> MGHHHHHHGSGSTNINLFSSYQLGELELPNRIVMAPLTRSRAGEGNVPHQLNAIYYGQRASAGLIIAEATQVTPQGQGYPHTPGIHSPEQVAGWKLVTDTVHQQGGRIFLQLWHVGRISHPDLQPDGGLPVAPSAIAPKGEVLTYEGKKPYVTPRALDTSEIPAIVEQYRQGAANALAAGFDGVEIHAANGYLIDQFLRDGTNKRTDEYGGAIENRARLLLEVTEAITSVWDSQRVGVRLSPLTTLNGCVDSHPLETFGYVAQALNRFNLSYLHIFEAIDADIRHGGTVVPTSHLRDRFTGTLIVNGGYTREKGDTVIANKAADLVAFGTLFISNPDLPERLEVNAPLNQADPTTFYGGGEKGYTDYPFLAVANK

To generalize this engineering approach for crystal contacts, a non-ADH-homologous enzyme was selected to apply the established strategies to the Nostoc sp. PCC 1720 ene reductase (NostocER). This oxidoreductase from the old yellow enzyme family (OYE, EC 1.6.99.1) catalyzes the trans-hydrogenations of activated alkenes, demonstrating its industrial relevance as a biocatalyst. As OYEs are strongly dependent on cost-intensive NADPH as a cofactor, Mähler et al. engineered NADH-accepting variants (NostocER1) by exchanging NostocER loop regions at cofactor-binding sites to ER loop regions from Achromobacter sp. JA81 and Acaryochloris marina with a higher NADH affinity. For this study, the NostocER1 Loop1,5 variant (NostocER1-L1,5) was selected as an example protein for the rational introduction of Lys–Glu interactions at crystal contacts to demonstrate the impact of rational single amino acid exchanges on the crystallizability of proteins and enhance protein crystallization.

Out of the nine tested NspER1-L1,5 mutants produced in E. coli, six crystallized, while four mutants revealed an increased propensity to crystallize in static µL-batch crystallization compared to the wild type: Q204K, Q350K, D352K, and T354K. The best-performing mutant Q204K was selected for upscaling, crystallizing faster than the wild type in a stirred batch crystallizer. In addition, crystallization of 3.75 g L−1 Q204K revealed an extended nucleation window toward lower protein concentrations for this mutant. Out of these seven, three mutants (43%) crystallized significantly better than the NspER1-L1,5 WT, as demonstrated by five different parameters defined for enhanced crystallizability (see Section 1): Q204K (5/5), D352K (2/5), and T354K (2/5). It is noteworthy that the nucleation window of Q204K (compared to the WT) not only extended to reduced protein and crystallization agent concentrations, but also to different buffers. After crystallization initiation (addition of the crystallization buffer to the protein solution), the protein concentration of mutant Q204K declined and dropped to 1.1 g L−1 within five hours. Subsequently, the protein concentration of mutant Q204K decreased significantly slower, and the equilibrium was reached at 0.4 g L−1 within 19.5 h with a crystal yield of 91.7%. Crystallization of NspER1-L1,5 mutant Q204K was successfully performed with up to 35% (w/v) HCP in static µL-batch experiments, whereas the WT did not crystallize. Mutants Q204K and Q350K crystallized in space group P212121, with the RMSD of the crystalline environment in this crystal packing indicating structural differences. The crystal contact at positions Q204K and Q350K both reveal an approximation of the intermolecular partners E89 (5.3 Å) and E27 (7.8 Å), respectively, compared to the WT.>[2x]MAHHHHHHVGTNTGGVLVITDTIIVKSGQTYDGKGIKIIAQGMGDGSQSENQKPIFKLEKGANLKNVIIG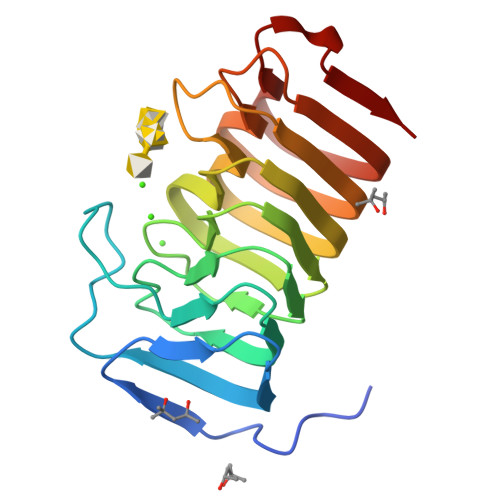APGCDGIHCYGDNVVENVVWEDVGEDALTVKSEGVVEVIGGSAKEAADAVFNLNAPCTFKVKNFTATNIGKLVRQNGNTTFKVVIYLEDVTLNNVKSCVAKSDSPVSELWYHNLNVNNCKTLFEFPSQSQIHQY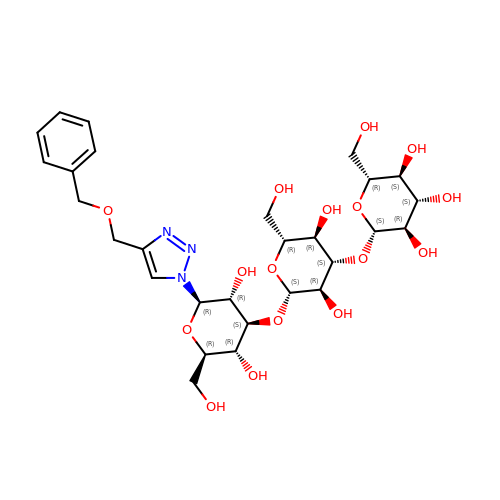(2~{R},3~{S},4~{S},5~{R},6~{S})-2-(hydroxymethyl)-6-[(2~{R},3~{R},4~{S},5~{R},6~{S})-2-(hydroxymethyl)-6-[(2~{R},3~{R},4~{S},5~{R},6~{R})-2-(hydroxymethyl)-3,5-bis(oxidanyl)-6-[4-(phenylmethoxymethyl)-1,2,3-triazol-1-yl]oxan-4-yl]oxy-3,5-bis(oxidanyl)oxan-4-yl]oxy-oxane-3,4,5-triol | C28 H41 N3 O16 | CUNJJKLJJLQYMH-ZJLPYKFYSA-N> GHMNMSQSQKIVLQPRSIVVPGELLAEGEFQIPWSPYILKINSKYYSTVVGLFDVKDTQFEVIPLEGSFYYPKINDIVIGLVEDVEIYGWVVDIKAPYKAYLPASNLLGRSINVGEDLRRYLDVGDYVIARIENFDRSIDPVLSVKGKDLGRVSNGIVIDIMPVKVPRVIGKNKSMYETLTSKSGCSIFVANNGRIWATCPSRFSEEILIEA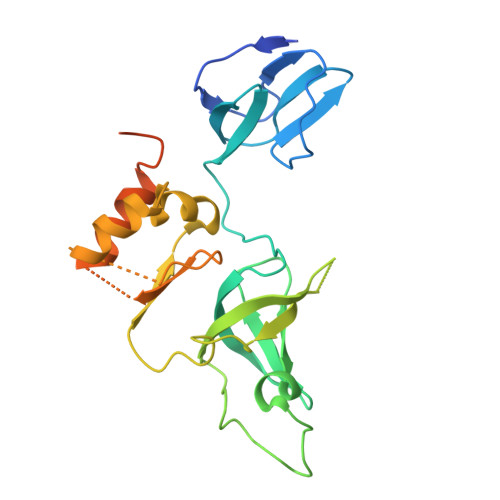IRKIENESHIKGLTDRIKQFIEEKLGERNASSGETKTNS>LDMSLNIHIKSGQDKWEVNVAPESTVLQFKEAI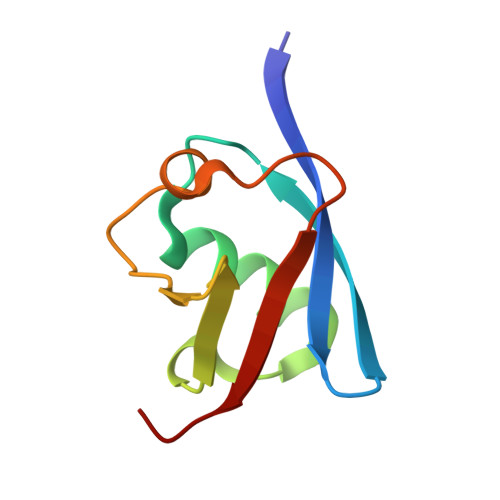NKANGIPVANQRLIYSGKILKDDQTVESYHIQDGHSVHLVKSQP[2x]> MKITLPKPFFFEGGNRAVLLLHGFTGSSADVRMLGRYLQKHGYTSLAPQYKGHAAPPEELTKTGPADWWQDVLDGYEELKAKGYDEIAVCGLSLGGVMSLRLSMHRPVKAVIPMCAPAYIKSEDVMYAGVTEYAREFKKREGKSVDEIEQEMAVFEPMPTLKDLQALLKETRDSLEDVYAPTLVVQARNDHMINTDSANIIHDGVSALQKELIWYENSGHVITLDKEKETLHQDIH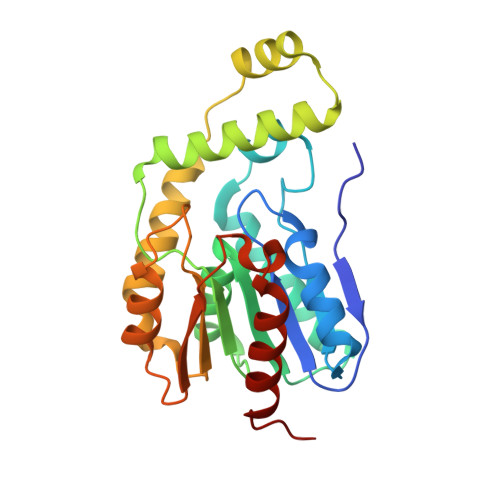EFLDGLNWSH>[6x]EEKDPLWLYKVLLTKGIEVWFDIKLEKYGIKRNNRVDYIAKSSLQQIVFEIIGKTPKNIAVPTYIGAYEPSKPEKWEEEGIKYINLFKPTPLMKVKPVKEMPEIVKNLLLNLFDYDAKSMGLFINWLAFIYQYKERTGVAWIFMGKQGTGKGLLVDLLKKIFEEHMSSNITDANLDSQFNPYLYNKLIVHLNEVSADNRKSRMLVKNRLKTWIT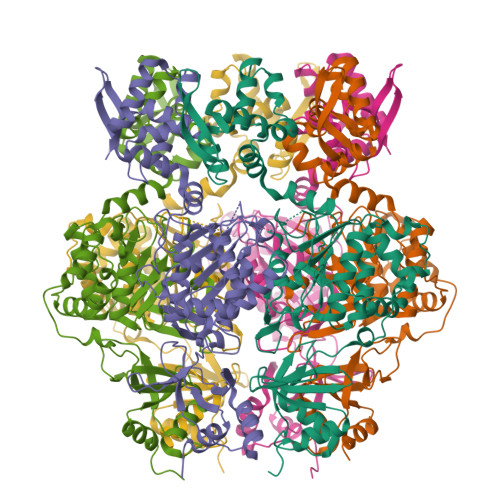DETLYINRKNMKEVEIKNFCNFIINSNETIPVDIEDSDRRFNVIECNNVLKEQEWWTTESYQEILNNAEGFAKYLAGIKVDRSKVNEVVMSEKKKAIVETTESVLKQIAKALTDRDIEWFLDNGLEGVVEKNIVNDFQWEELQEAITTGVIPNKYLMIIVEQILGDSKTITWIKRNIITPYQVGETTVVKMAGKPIRAIVVG Lamins represent a distinct class within the intermediate filament (IF) protein family. Lamin A (LA) and its splice variant lamin C as well as two closely related lamins B1 and B2 jointly form the lamina, a meshwork of ~3.5-nm-thick filaments located at the inner side of the nuclear envelope. Like for the whole IF family, the basic constitutive unit of the lamin filament is a rod-like dimer which results from a parallel coiled-coil (CC) structure. In line with this, the primary structure of lamins reveals a central α-helical domain responsible for the CC formation which is flanked by non-helical N- and C-terminal domains called the head and the tail respectively.

In addition, a construct comprising residues 1–49 of the Gp7 protein (N-terminal cap) fused by LA residues 327–403 was prepared. The last chimera additionally included a F40C point mutation, located at heptad repeat position ‘d’ within the Gp7 cap. This mutation was made to introduce a disulphide bridge in order to facilitate experimental crystallographic phasing, since the initial location of a disulphide from anomalous diffraction data is substantially easier than of isolated sulphurs. The crystal structure of the Gp7F40C-LA 327-403 fusion construct was established to 2.9 Å resolution. To this end, experimental phasing on sulphur atoms could be used, which had been facilitated by an engineered disulphide bridge in the dimeric Gp7F40C cap. Crystallographic data reveal good electron density for the capping motif and the lamin part up to residue 381, i.e., exactly the predicted end of the rod domain. The tail domain part (residues 382–403) is disordered in the crystals. While the LA 305-387 structure becomes increasingly disordered towards its N-terminus, our fusion with the Gp7F40C cap provides for a proper stabilization of the LA sequence. As a result, the CC geometry of Gp7F40C-LA 327-403 reveals an unwinding that is in line with theoretical expectations for a stutter. First, the capping motifs used (and especially the Gp7F40C cap that had been additionally stabilized by a disulphide bridge) provide for the correct assembly of dimeric, registered CCs even for short lamin fragments.

> GMPLKPEEHEDILNKLLDPELAQSERTEALQQLRVNYGSCVSEYNDLTKSLARERDTSRRLLAEKEREMAEMRARMQQQLDEYQELLDIKLALDMEIHAYRKLLEGEEERLRLSPSPTSQRSRGRAS> MNEHYTESDIKRNHKTEKNKTEKEKFKDSINNLVKTEFTNETLDKIQQTQDLLKKIPKDVLEIYSELGGEIYFTDIDLVEHKELQDLSEEEKNSMNSRGEKVPFASRFVFEKKRETPKLIINIKDYAINSEQSKEVYYEIGKGISLDIISKDKSLDPEFLNLIKSLSDDSDSSDLLFSQKFKEKLELNNKSIDINFIKENLTEFQHAFSLAFSYYFAPDHRTVLELYAPDMFEYMNKLEKGGFEKISESLKKEGVEKDRIDVLKGEKALKASGLVPEHADAFKKIARELNTYILFRPVNKLATNLIKSGVATKGLNVHGKSSDWGPVAGYIPFDQDLSKK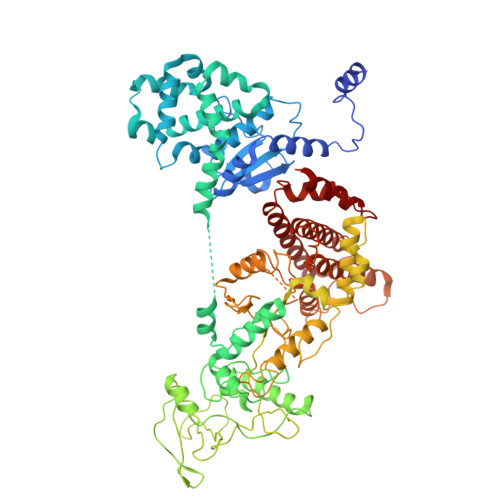HGQQLAVEKGNLENKKSITEHEGEIGKIPLKLDHLRIEELKENGIILKGKKEIDNGKKYYLLESNNQVYEFRISDENNEVQYKTKEGKITVLGEKFNWRNIEVMAKNVEGVLKPLTADYDLFALAPSLTEIKKQIPQKEWDKVVNTPNSLEKQKGVTNLLIKYGIERKPDSTKGTLSNWQKQMLDRLNEAVKYTGYTGGDVVNHGTEQDNEEFPEKDNEIFIINPEGEFILTKNWEMTGRFIEKNITGKDYLYYFNRSYNKIAPGNKAYIEWTDPITKAKINTIPTSAEFIKNLSSIRRSSNVGVYKDSGDKDEFAKKESVKKIAGYLSDYYNSANHIFSQEKKRKISIFRGIQAYNEIENVLKSKQIAPEYKNYFQYLKERITNQVQLLLTHQKSNIEFKLLYKQLNFTENETDNFEVFQKIIDEK>[4x]SIYLPLPQADDQYTPYFVYNFQGERVSTTETGVFCLAAIPAATTSSRYNNQITIPSIGYRNASGTGTL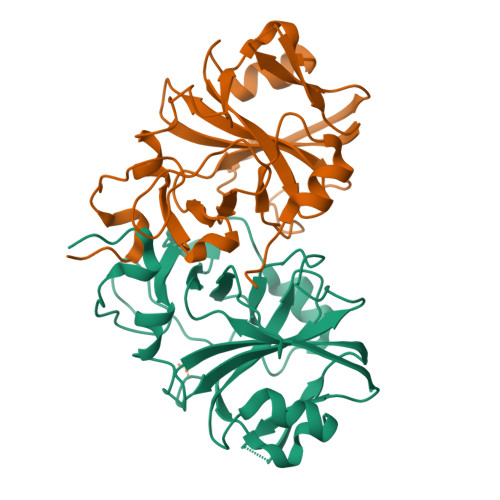FLLDAASWWNILDVTQTGVLFGQPRLGVGVMQTMKTLKQHIKDYTEPAIQKYYPGTTNLDEQLKQRLNLAEGDPVISMGDTNGRRAALFYRTSDEKYILFFSTTEDPGAQYQNLKMLYFWNWSYSDTKQQFLDHLRTVQF> GGCCGAA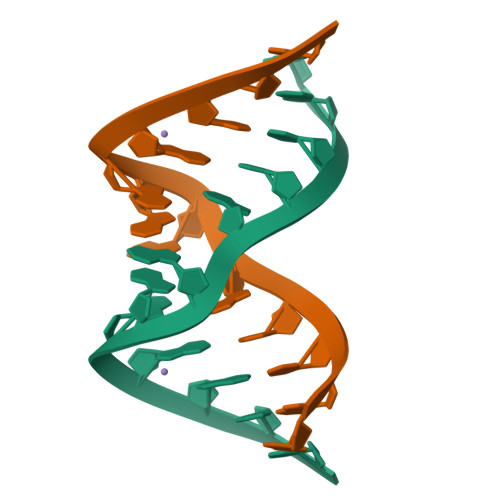AGGCC>MKVSVIGATGYTGYELVKILANHPEFEIAALVSETYADKMFSDVYPRLRSICDVVITGRDYDAVAEISDAVFLCLPHAAAQDAAAFFYEKGLKVVDFSADFRLKDKKLYEATYKVDHTYPDLLRKAVYGLPEIFEVDIKKAELVANPGCYPTSVITPLYPLLKAGLISPEGIIADSKVGVTVAGRKADIAYSFCECNEDFRPYAIFSHRHNPEINEVLKETGKETNVLFTPHIIPASKGIESTIYTKTTAGLAEISACLKDFYRERRCVRIYDNGHIPSTADVTDTNFIDIGLFVKGERLIIVSCIDNLIKGSSGMAVQNMNLMCGFDDTLGILLEHHHHHH[4x]

Here, we seek to establish the direct reduction of formyl phosphate into formaldehyde through developing a new-to-nature enzyme, formyl phosphate reductase (FPR). We identify promiscuous FPR activity in four enzyme families and present one homolog of N-acetyl-γ-glutamyl phosphate (NAGP) reductase from Denitrovibrio acetiphilus (DaArgC) that produces relevant levels of formaldehyde. The ArgC active site can be divided into three parts, the NADPH-binding domain, the catalytic site, and a substrate-binding channel. The catalytic site consists of catalytically active C149 and the HRH motif (residues 208-210) responsible for binding the phosphate and carbonyl group of the substrate (gray labeling in Fig. 3a).

Round 1 of mutagenesis resulted in variant DaArgC G182V (DaArgC1), which was followed by an S178V substitution in round 2 of mutagenesis (DaArgC2). Using double variant DaArgC2 as a template, we discovered a L233I substitution that showed an additional beneficial effect, resulting in triple variant DaArgC3. Using a semi-rational enzyme engineering approach, we create a triple substitution variant of the enzyme (DaArgC3) that shows a complete loss of the native enzyme activity (i.e., NAGP reduction), a 300-fold shift in specificity towards formyl phosphate, and a decreased side reactivity with acetyl phosphate. Across all substrate concentrations, DaArgC3 showed a fourfold improved formaldehyde productivity over wild-type (WT) DaArgC in vivo. Variants DaArgC1, DaArgC2 and DaArgC3 showed similar turnover numbers (0.1–0.2 s−1), but were already saturated at apparent Km (formyl phosphate) values around 20-30 mM, indicating that they performed better at formyl phosphate concentrations that are physiologically more relevant in vivo. The apparent Km for NADH (~0.3 mM) was approximately sixfold higher compared to NADPH, while the specific activities were at about 50% of the activity with NADPH (~0.1 s−1), indicating that variants DaArgC1-C3 had evolved to also accept NADH as redox cofactor, which they could additionally access in vivo besides NADPH. When we re-established the glycine residue at position 182 in DaArgC2 and DaArgC3 (creating variants DaArgC2* and DaArgC3*), NADPH selectivity of the variants was fully restored, indicating that the glycine to valine substitution was responsible for the observed cofactor flexibility. Solving the crystal structure of DaArgC3 suggested that the position of residues T9, S33, E34 and T35 (numbering according to mtArgC29) that interact with the 2′ phosphate of NADPH was not significantly affected by the G182V mutation. However, we noted that G182 lies within the conserved GAG motif of the substrate-binding channel (residues 182–184) and is flanked by two amino acids, T181 and R185, that form hydrogen bonds to the nicotinamide group and the diphosphate of NADPH, respectively.>[2x]HHHHHHMEPACKYDFATSVLFTEAELHTRMRGVAQRIADDYSNCNLKPLENPLVIVSVLKGSFVFTADMVRILGDFGVPTRVEFLRASSYGHDTKSCGRVDVKADGLCDIRGKHVLVLEDILDTALTLREVVDSLKKSEPASIKTLVAIDKPGGRKIPFTAEYVVADVPNVFVVGYGLDYDQSYREVRDVVILKPSVYETWGKELERRKAAGEAKR

One potential new drug target is 6-oxopurine phosphoribosyltransferase (PRTase), an enzyme central to the purine salvage pathway and whose activity is critical for the production of the nucleotides (GMP and IMP) required for DNA/RNA synthesis within this protozoan parasite. For example, T. brucei has three 6-oxopurine PRTase isoforms whereas there is only one 6-oxopurine PRTase in humans. These enzymes catalyze the transfer of the ribose 5'-phosphate moiety from 5-phospho-α-D-ribosyl-1-pyrophosphate (PRib-PP) to their respective purine bases (hypoxanthine, guanine or xanthine). Here, we show that two of the three T. brucei isoforms of the 6-oxopurine PRTases are identified as HGPRTs as a reflection of their substrate preference for hypoxanthine and guanine and the third isoform is identified as HGXPRT reflecting that it uses all three naturally occurring bases. In both enzymes, the active site is situated at the interface of two domains referred to as the hood and core and is primarily comprised of three pockets identified as the purine base binding pocket, the 5′-phosphate binding pocket and the pyrophosphate (PPi) binding pocket.

To explain the mode of binding of the ANPs, crystal structures of HGPRT-I in complex with compounds 1, 2, 6 and 7, and HGXPRT in complex with compounds 2 and 7 were determined. In the HGPRT-I.6 complex the PPi binding site is occupied by the phosphonate connected to the attachment. This phosphonate interacts with the side chain atoms of D114, D173, R179 and two water molecules. In this complex the side chain of L53 points inwards towards the active site and the peptide bond between L53-K54 is in the trans conformation. This allows L53 to form hydrophobic interactions with three carbon atoms from the linker and attachments. However, in other crystal structures of HGPRT-I (e.g. in complex with GMP and IMP) the peptide bond between L53 and K54 can exist in the cis conformation, resulting in the side-chain of L53 being rotated out of the active site, allowing space for PRib-PP to bind. In addition, in HGPRT-I the L53-K54 peptide bond is in trans conformation and the side chain of L53 points into the active site, whereas in the human enzyme when compound 6 binds the equivalent peptide bond is in the cis conformation. Further, in the crystal structure of the human enzyme a sulphate ion fills the PPi binding pocket, whereas there is no sulphate in the HGPRT-I and HGXPRT structures. Compounds 3 and 6 are the most broadly effective inhibitors tested so far with Ki values lower than 1 μM for all three enzymes.The SLAC1 homolog, HiTehA, although not completely biochemically characterized, is identified as a transporter protein involved in tellurite resistance and adaptation to environmental stresses, highlighting its role in bacterial survival through regulating solute concentrations. HiTehA is a trimeric protein; each monomer comprises 10 transmembrane helices (TMs) connected by short extracellular loops and slightly longer intracellular loops; a short helix is part of the loop connecting TM2. The ion channel architecture features a distinctive organization: the pore-forming helices are positioned at odd-numbered TMs, while the even TMs collectively form an outer shell. This outer shell contributes significantly to the overall stability and functionality of the channel, potentially playing a pivotal role in sensing environmental changes, responding to stimuli, and regulating the opening and closing dynamics of the channels.

We successfully elucidated the structures of all four samples with an average resolution of 3 Å. The HiTehA purified using GDN achieved the highest resolution of 2.9 Å, followed by those purified with DDM and LMNG at resolutions of 3.1 Å, and OG at 3.2 Å, as detailed in Table 1 and Figure S1. The four structures of HiTehA closely align, revealing a minimal root-mean-square deviation (r.m.s.d.) of 0.13 Å for all atoms, except for the sample purified in DDM, which showed a slightly higher deviation of 0.26 Å. In general, the structural integrity of the trimeric arrangement remains unaffected using four different detergents during protein purification. Remarkably, none of the detergents tested appear to induce any significant alteration in the position of the gating Phe262 located on TM9. This observation underscores the robustness of the trimeric structure and the stability of key functional elements within HiTehA, even under varying detergent conditions. The identification of a linear density within the channel cavity across all detergent conditions suggests this cavity can be occupied either by detergent molecules or by other hydrophobic molecules such as co-purified lipids.

>[3x]MNITKPFPLPTGYFGIPLGLAALSLAWFHLENLFPAARMVSDVLGIVASAVWILFILMYAYKLRYYFEEVRAEYHSPVRFSFIALIPITTMLVGDILYRWNPLIAEVLIWIGTIGQLLFSTLRVSELWQGGVFEQKSTHPSFYLPAVAANFTSASSLALLGYHDLGYLFFGAGMIAWIIFEPVLLQHLRISSLEPQFRATMGIVLAPAFVCVSAYLSINHGEVDTLAKILWGYGFLQLFFLLRLFPWIVEKGLNIGLWAFSFGLASMANSATAFYHGNVLQGVSIFAFVFSNVMIGLLVLMTIYKLTKGQFFLK> MTVATTKTREYAEIVYKIAQGFVLSKLSSKHDLQW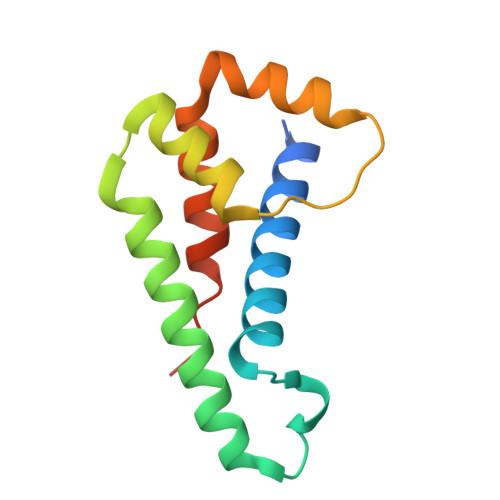SKCKGNPKLEREYNDKKEKVVNEAFLAIRSRTEKQAFIDYFVSTLYPHVRQDEFVDFAQKLFQDTDEIRSLTLLALSSQYPIKRQGETE>GAEFMDIDKDAFAAKEQALKQERPEGLVGGLQPKKLVNLENLVFDQGNHLMTNPRVRMPEGTTKRVFKGYEEIHVPPPKKRSDPTDQNIPVTELPEWARIPFNTTKTLNKIQSKCFPTAFLDDGNMLVCAPTGSGKTNVAMLTMLREIGKNRNEKGEIDLDAFKIVYIAPLKALVQEQVGNFGKRLEPYGIKVSELTGDRQLTKQQISETQVIVTTPEKWDVITRKATDISYTNLVRLIIIDEIHLLHDDRGPVLESIVSRTIRRTEQTGEPVRIIGLSATLPNYRDVASFLRVDFEKGLFYFDGSYRPCPLRQEFIGVTDKKAIKQLKTMNDITYQKVLEHVGQNRNQMLIFVHSRKETAKTAKYIRDKALEMDTINQILKHDAGTREVLQEAASSVNNTDLKDLLPYGFGIHHAGMSRADRTDVEDLFASGHIQVLVCTATLAWGVNLPAHTVIIKGTQVYSPEKGSWVELSPQDVLQMLGRAGRPQYDTYGEGIIITTQGEIPYYLSLLNQQLPIESQLVSKLVDSLNAEIVLGNVRNRDEGVEWLGYTYLFVRMLRSPGLYSVGAEYEDDVALEQKRVDLIHSAAMVLKKSNLIKYDEKTGKMQATELGRIASHYYISHESMDTYNKLIHPAMNDVELFRVFAQSGEFKYIPVRQEEKLELAKLLARVPIPVKESIEEPTAKINVLLQAYISRLKLEGLALMADMVYVTQSAGRILRAIFEICLKKGWASVAKLALNMCKMAEKRMWPTMSPLRQYPTCPAEIIKKAERMDVPWSSYFDLDPPRMGELLGMPKAGKTVCALVSKFPRVEIQGNVQPMTRSMLRIELTITPNFQWDVELHGVTESFWILVEDCDGEEILFHDVFILRKDLAE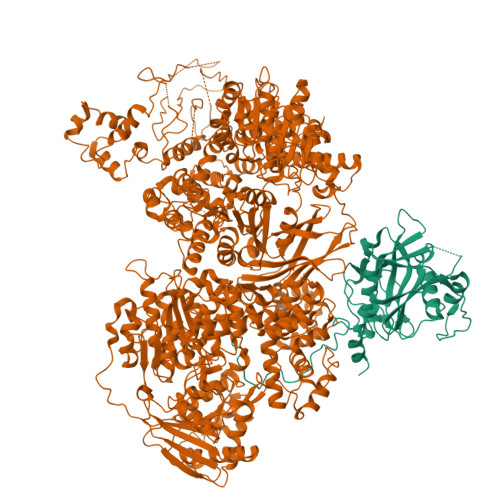AEENEHTVEFTVPISEPMPPNYFISVISDRWMHSETRMPVSFQKLILPERFPPHTELLDLQPLPVSALKAKDYAALYPNWQQFNKIQTQTFNSLYNTDNNVLVAAPTGSGKTVCAEFALLRHWAKKDAGRAVYIAPFQELVDLRFQDWQKRLSHLRGGKEIVKLTGETTTDLKLLEQGDLILATPLQWDVLSRQWKRRKNVQTVELFIADDLHMLGGQMGYIYEIVVSRMHFIRTQTELPMRIVGLSVSLANARDIGEWIDAKKHDIYNFSPHVRPVPLELHIQSYTIPHFPSLMLAMAKPTYLAITQLSPDQPAIVFVPSRKQTRATARDLLTACLADDDEDRFLHVEVDQIRKLLDHVQEEALAEALSHGVGYYHEALSQSDKRIVKHLYNNGAIQVLIASRDVCWELDFTAHLVVVMGTQFFEGKEHRYIDYPLSEVLQMFGKALQPSKDGRSRGVLMLPAVKREYYKKFLNEALPVESHLHNFLPDAFVTEISTKMIESGEDAINWATFTYFYRRLLANPSYYGLQDPTHDGLSQYLSDLVETTLKQLSDARIIEMDEDEGTVAPLNAAMIAAYYNISYMTMEMFLLSLSHKSKLRTILEIVTAATEFESIQTRRHEEGILKRIYDHVPVKMNNPVWDSAHFKAFVLVQAHFSRMNLPIDLAKDQEVILQKILSLLSAIVDILSSEGHLNALNAMEMSQMVVQAMWDRDSPLKQIPNFTPEVVKVANKYGINDIFDFMEQMNPEENPNYASLVKDLGLTQAQLAQAANFTNNKYPDITLEFEVDDPDNIRAGEPAYLKIHIERELEEDEEFDPTVHAPFYPGKKSENWWLVVGEESTKTLLAIKRVTVGKELNVKLEFVVPSPGKHDLKLFLMSDSYVGVDQDPSFSVNVAEG[4x];>[4x]GAMQQTFASKTEWRTRAIATSNLRTRANNMYVAPVDNDVDDITYVMPKNILKKFITIADLRVQVAGFLYGCSPADNDQVKEIRCIVMVPQIGGNRSVQLPQHLPQHEMLKGLEPLGLIHTMAGNELPYMSPADVTTHAKLVDAHPSWKNQNTLTVTVAFTPGSVSLSAWALTPLGYKWGVENKDPNVDNPQGFTTTMGERRQLLLSDKFKGFFLVPDTGKWNYSFMGSSFSGIEKKPYHVKLDTPLPFYSEQHRPIHFTSFNELEDIWVDRADNFA>[4x]MHHHHHHLPNITILATGGTIAGGGDSATKSNYTVGKVGVENLVNAVPQLKDIANVKGEQVVNIGSQDMNDNVWLTLAKKIN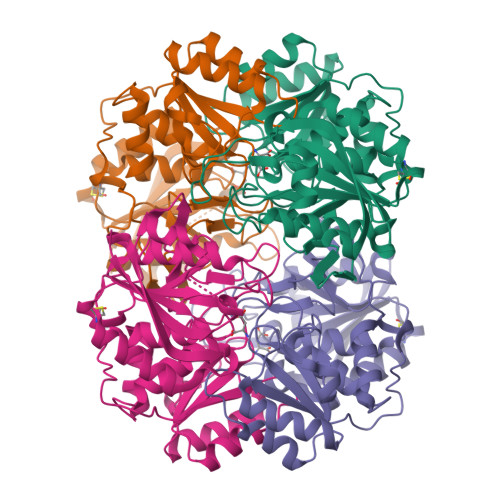TDCDKTDGFVITHGTDTMEETAYFLDLTVKCDKPVVMVGAMRPSTSMSADGPFNLYNAVVTAADKASANRGVLVVMNDTVLDGRDVTMTNTTDVATFKSVNYGPLGYIHNGKIDYQRTPARKHTSDTPFDVSKLNELPKVGIVYNYANASDLPAKALVDAGYDGIVSAGVGNGNLYKSVFDTLATAAKTGTAVVRSSRVPTGATTQDAEVDDAKYGFVASGTLNPQKARVLLQLALTQTKDPQQIQQIFNQY> GGVDRWPEYYPETGRDIWIDSVMRQEYLWYRDMPSPAAPDYFQKPEAFLKKAVASMDNGFSKIDSLLDEPIPSYGFDYTLYKVLDNDTAYNALISYVVPGSPAEEAGLQRGHWIMMMNGDYITKKVESELLQGSTRQLQIGVYKEVVGEDGEVTGGVVPIGETTMPASRSLVDKPVHRFEIIPWNGKKVGYLMYNEFKAGPTTD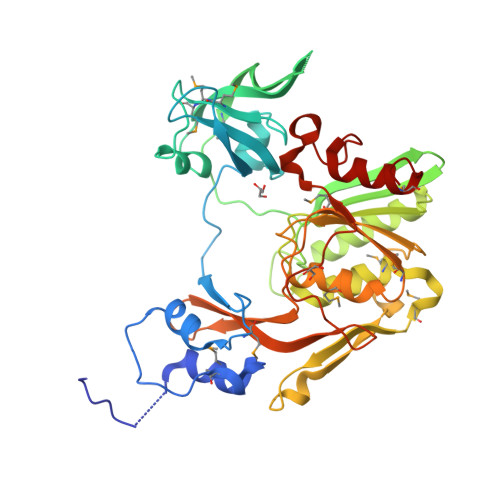SQAYNDDLRRAFRDFQTGGVNEFVLDLRYNTGGSLDCAQLLCTMLAPADKMNQLLALLRYSDKRVEANQDLTFNPELIQSGANLNLSTVYVLTTNATRGAAEMVINCLNPYMKVVLIGTKTAGEYVATKPFVHPTDRFILNLVVCNVYNAEEKSDYATGFKPTYEYNEDSYLSTYLPFGNTNETLLNAALKIMSGITDK> MAHYPTRLKTRKTYSWVGRPLLDRKLHYQTYREMCVKTEGCSTEIHIQIGQFVLIEGDDDENPYVAKLLELFEDDSDPPPKKRARVQWFVRFCEVPACKRHLLGRKPGAQEIFWYDYPACDSNINAETIIGLVRVIPLAPKDVVPTNLKNEKTLFVKLSWNEKKFRPLSSELFAELNKPQESAAKCQKPVRAKSKSAESPSWTPAEHVAKRIESRHSASKSRQTPTHPLTPRARKRLELGNLGNPQMSQQTSCASLDSPGRIKRKVAFSEITSPSKRSQPDKLQTLSPALKAPEKTRETGLSYTEDDKKASPEHRIILRTRIAASKTIDIREERTLTPISGGQRSSVVPSVILKPENIKKRDAKEAKAQNEATSTPHRIRRKSSVLTMNRIRQQLRFLGNSKSDQEEKEILPAAEISDSSSDEEEASTPPLPRRAPRTVSRNLRSSLKSSLHTLTKVPKKSLKPRTPRCAAPQIRSRSLAAQEPASVLEEARLRLHVSAVPESLPCREQEFQDIYNFVESKLLDHTGGCMYISGVPGTGKTATVHEVIRCLQQAAQANDVPPFQYIEVNGMKLTEPHQVYVQILQKLTGQKATANHAAELLAKQFCTRGSPQETTVLLVDELDLLWT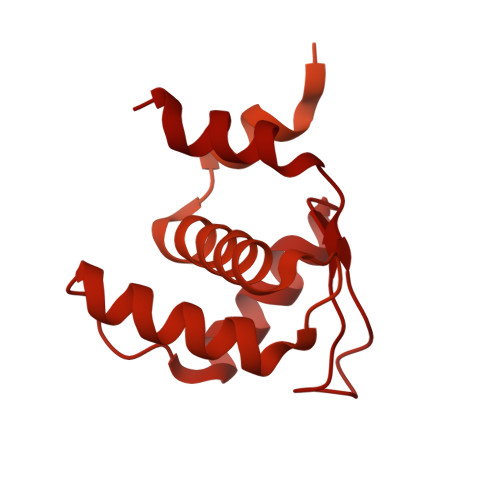HKQDIMYNLFDWPTHKEARLVVLAIANTMDLPERIMMNRVSSRLGLTRMCFQPYTYSQLQQILRSRLKHLKAFEDDAIQLVARKVAALSGDARRCLDICRRATEICEFSQQKPDSPGLVTIAHSMEAVDEMFSSSYITAIKNSSVLEQSFLRAILAEFRRSGLEEATFQQIYSQHVALCRMEGLPYPTMSETMAVCSHLGSCRLLLVEPSRNDLLLRVRLNVSQDDVLYALKDE> MNDIYARRLAQATMFHQLMRCHGTLWAATQVTKEQMDYNFIREEFMRVNGRRAM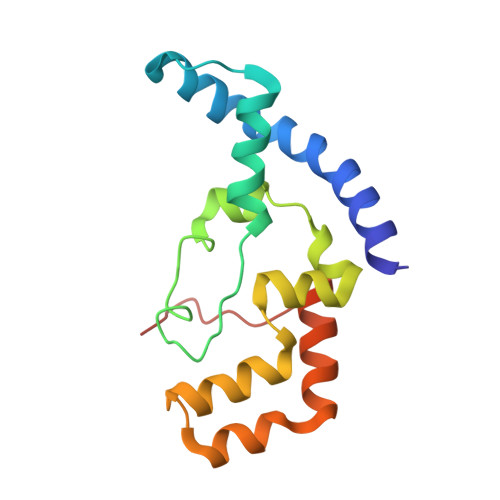PLLLGAAANENLHQLHLSHLSEHCAWGESARALAVQRQTPLSQRVAALGRMAETIHQVKTASTVQNLFNEQISCMEGISSFEEEPLIEGE>MRGSHHHHHHGLVPRGSMQNPRTVSDTKRAFYAAHTRPIHSIYRRFIEELLVEIHLLRVNVDFRYSPLFALGVVTAFDQFMEGYQPEGDRDRIFHALCVAEEMNPQQLKEDAASWQQYQGRPLSQILDELNSGQPSAPLNSLNHTGKYSRLHAVGLYAFLQELAGEVTIHLNETLDQLAPVIP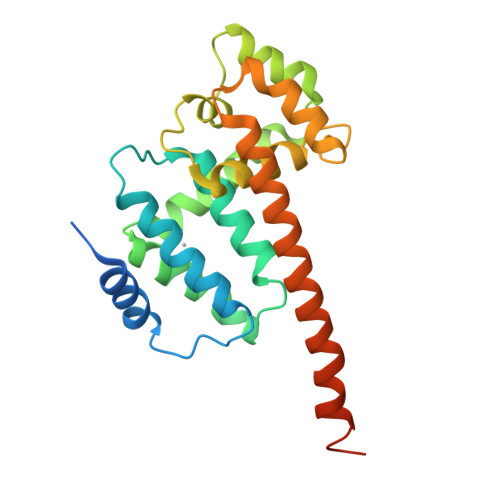LPIEKVKRDLELYRSNLDKINQARSLMKELVEQERKRRAQQTSAPPAVDASSDAPA[7x]>MVANPEHYIKHPLQNRWALWFFKNDKSKTWQANLRLISKFDTVEDFWALYNHIQLSSNLMPGCDYSLFKDGIEPMWEDEKNKRGGRWLITLNKQQRRSDLDRFWLETLLCLIGESFDDYSDDVCGAVVNVRAKGDKIAIWTTECENREAVTHIGRVYKERLGLPPKIVIGYQSHADTATKSGSTTKNRFVV[2x];>XRYSRL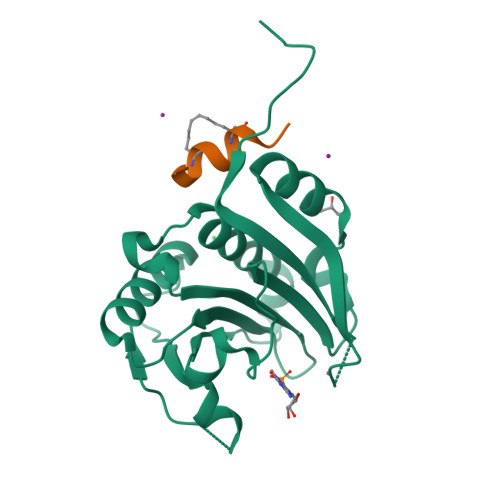QLLLLFRX[2x]>NLMQFELLIMKVAGRSGIVWYSDYGCFCGKGGHGRPQDATDRCCFVHDCCYGKVNGCDPKEDFYRYSSNNGDIVCEANNPCTKEICECDKAAAICFRDNKDTYDNKYWNIPMESCQESE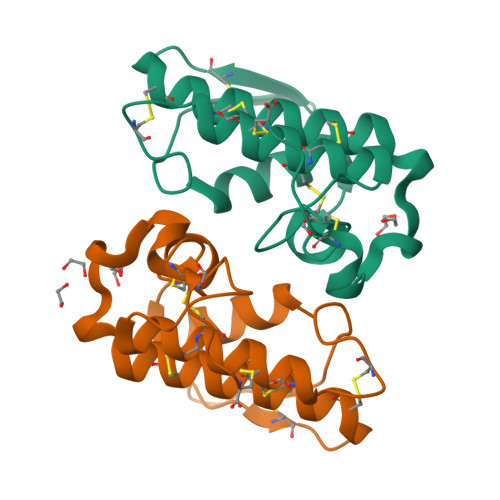PC[2x]> GPYLQILEQPKQRGFRFRYVCEGPSHGGLPGASSEKNKKSYPQVKICNYVGPAKVIVQLVTNGKNIHLHAHSLVGKHCEDGV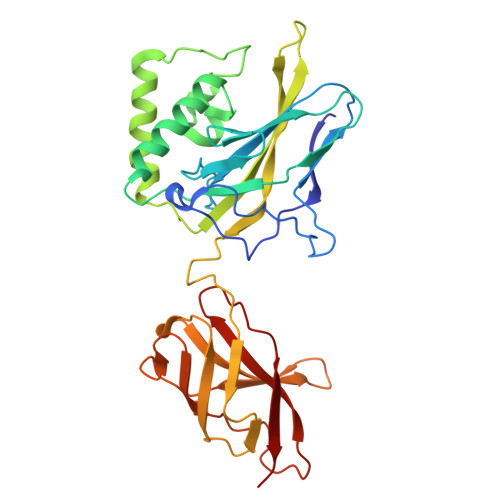CTVTAGPKDMVVGFANLGILHVTKKKVFETLEARMTEACIRGYNPGLLVHSDLAYLQAEGGGDRQLTDREKEIIRQAAVQQTKEMDLSVVRLMFTAFLPDSTGSFTRRLEPVVSDAIYDSKAPNASNLKIVRMDRTAGCVTGGEEIYLLCDKVQKDDIQIRFYEEEENGGVWEGFGDFSPTDVHRQFAIVFKTPKYKDVNITKPASVFVQLRRKSDLETSEPKPFLYYPE>UUGCGUCACAC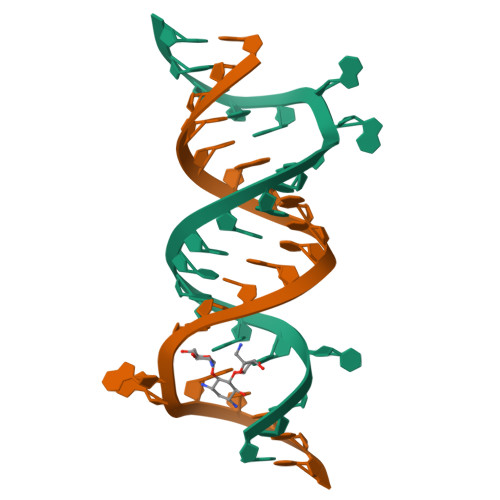CGGUGAAGUCGC[2x]N-{(1R,2R)-2-[(4aS,7aR)-2-amino-4a,5-dihydro-4H-furo[3,4-d][1,3]thiazin-7a(7H)-yl]cyclopropyl}-5-fluoropyridine-2-carboxamide | C15 H17 F N4 O2 S | 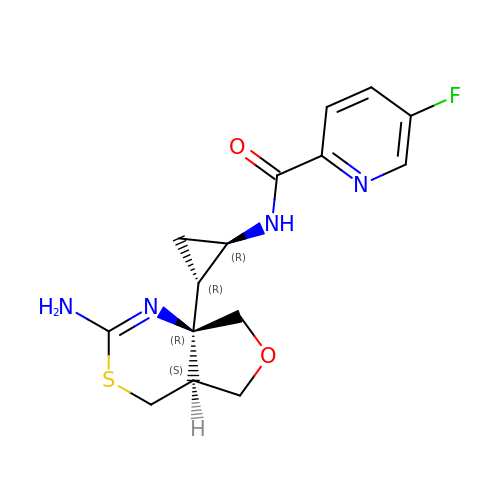OWWIYTVWTQBRDL-RAAPYIGPSA-N> MSFRYTNGLVGALKHRMMLESSHRELVRRRFTGHCRGVEVVCSGYGTVLAVRLVDKTVWEPFYRKGHPSPSGADMDSAPPSSHAEGTPVGGQSAAPLDFERIAESIKAALWDATRKIRSAKEAALNRSLSHNQQLRAQAHLEHWYDEDANTLQPLAFEALKHEAATPWMQFVQFGKYKHAAAVMHSESGGKTSEAFTGETKRAGADNEEGPCVTALDEKDVDPTSIPIGSVHPLFLPALIQFESRVDNSLNDDAIR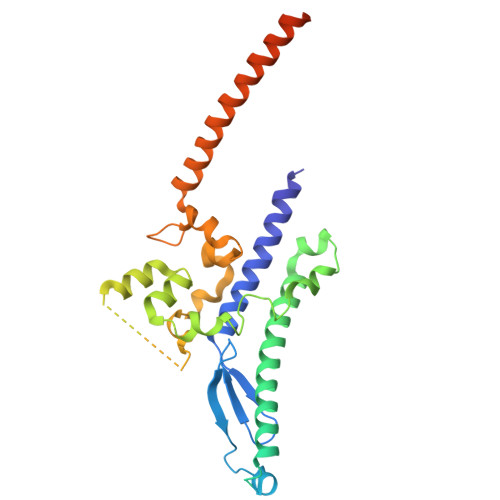QEQRREMSRDEQLFWERVELIRKGQVATIKGGHKRDYADEAAVASDNAVDKVQLRFTQ>[2x]MSELEKAMVALIDVFHQYSGREGDKHKLKKSE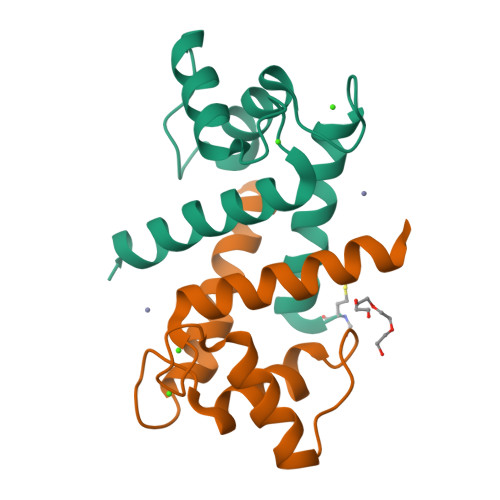LKELINNELSHFLEEIKEQEVVDKVMETLDNDGDGECDFQEFMAFVAMVTTACHEFFEHE>IKPSNILPVTVYDQHGFRILFHFARDPLPGRSDVLVVVVSMLSTAPQPIRNIVFQSAVPKVMKVKLQPPSGTELPAFNPIVHPSAITQVLLLANPQKEKVRLRYKLTFTMGDQTYNEMGDVDQFPPPETWGSL[4x];>SLDGTGWNSFQSS[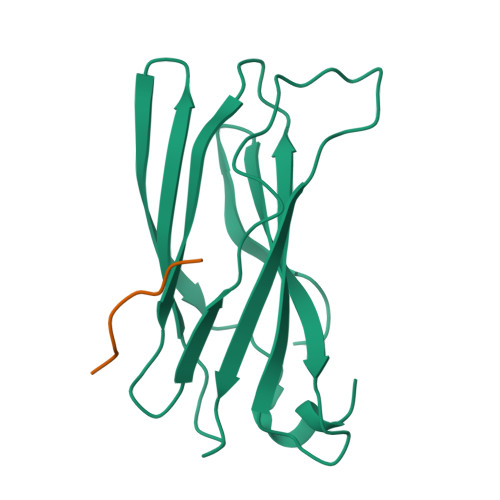2x]5-(4-fluorophenyl)-2,3-dihydroxy-N-(4-thieno[3,2-c]pyridin-2-ylbutyl)benzamide | C24 H21 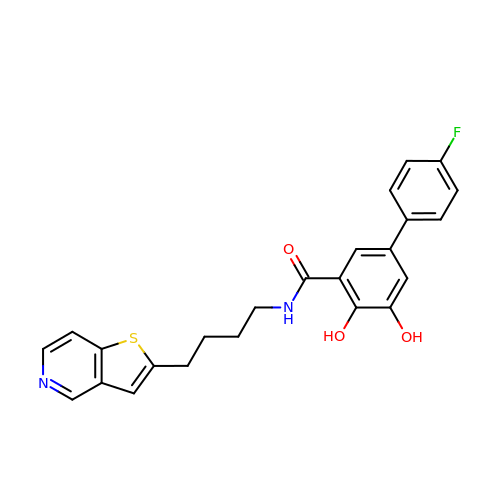F N2 O3 S | XWFQNEQLXCLGOK-UHFFFAOYSA-N>[6x]MSDSVFNKDERIMDLVSKHYNVELCAANLYFHLATVSKALGYDNVAAFFVKMGSDKQSAHMSRLVKYMMKVDSILKINQISVPELVSFETIQEVLDAALKMESKVRES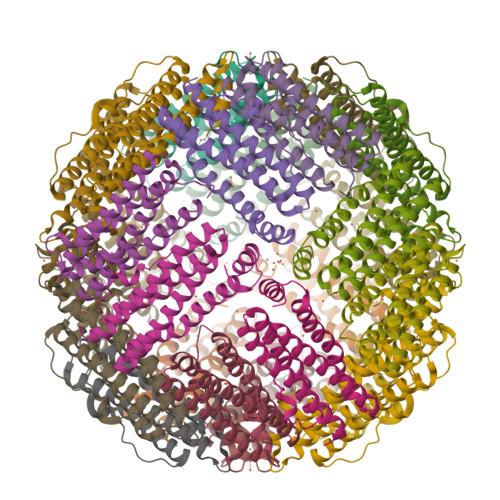VKNVTEISLLAKDFETFERMQWFVKDSIEDLEEISDVWTYVHSPNVNLINIENIVGKKLKKSEYDDDHDED> MHYRISFIFVTFICLFCFAATGFTQNTNHHHHHHHTDEDSKPVILYSGTPKKYEIADIKVEGVKNYEDYVLIGLSGLSVGQTITVPGDEITGAIKRYWKHGLFSNVQITAEKIEGNKIWLKISLTQRPRIADVRYHGVKKSERTDFESKLGMVKGMQITPNTVDRAKTL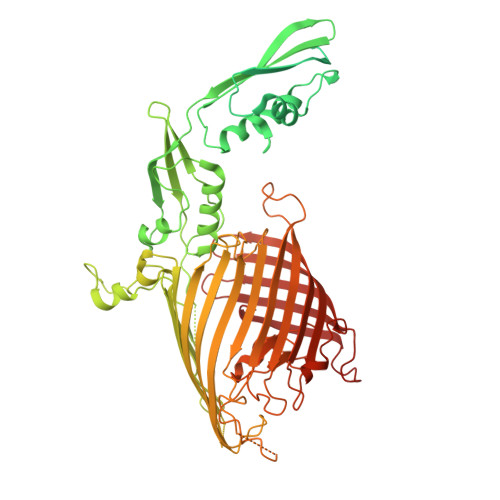IKRYFDDKGFKNAEVIIAQKDDPSNENQVIVDIDIDKKEKIKVHAIHITGNSAIKTSKLKKVMKKTNEKGKLLNLFRTKKFVPENFEADKQLIIDKYNELGYRDAMIVKDSVAQYDEKTVDVYMDIDEGQKYYLRNVTWVGNTLYPSEQLNFLLRMKKGDVYNQKLLGERTSTDDDAIGNLYYNNGYLFYNLDPVEVNIVGDSIDLEMRIYEGRQATINKINISGNDRLYENVVRRELRIRPGQLFSKDDLMRSLREIQQMGHFDPEKLQPDIQPDPVNGTVDIGLPLTSKANDQVEFSAGWGQTGIIGKLSLKFTNFSVANLLRPGENYRGILPQGDGQTLTISGQTNAKYYQSYSISFFDPWFGGKRPNSLSVSAFFSVQTDISSRYYNSSYFNNYYNSMYSGYGGYGMYNYGNYNNYENYYDPDKSIKMWGLSLGWGKRLKWPDDYFTLSAELAYQRYNLKDWQYFPVTNGKCNDLSLSLTLARNSIDNPIFPRTGSDFSLSVQLTPPYSLFDGKDYKGYFYDPTDDRGITQDNMNKLHRWVEYHKWKFKAKTYTPLMDYIAHPKCLVLMTRTEFGLLGHYNKYKKSPFGTFDVGGDGMTGYSSYATESIALRGYENSSLTPYGKEGYAYARLGIELRYPLMLETSTNIYVLGFLEAGNAWHDISKFNPFDLKRSAGIGVRIFLPMIGMMGIDWGYGFDKINGSKEYGGSQFHFILGQEF>[2x]SDNDPLVVNTDKGRIRGITVDAPSGKKVDVWLGIPYAQPPVGPLRFRHPRPAEKWTGVLNTTTPPNSCVQIVDTVFGDFPGATMWNPNTPLSEDCLYINVVAPRPRPKNAAVMLWIFGGSFYSGTATLDVYDHRALASEENVIVVSLQYRVASLGFLFLGTPEAPGNAGLFDQNLALRWVRDNIHRFGGDPSRVTLFGESAGAVSVSLHLLSALSRDLFQRAILQSGSPTAPWALVSREEATLRALRLAEAVGCPHEPSKLSDAVECLRGKDPHVLVNNEWGTLGICEFPFVPVVDGAFLDETPQRSLASGRFKKTEILTGSNTEEGYYFIIYYLTELLRKEEGVTVTREEFLQAVRELNPYVNGAARQAIVFEYTDWTEPDNPNSNRDALDKMVGDYHFTCNVNEFAQRYAEEGNNVYMYLYTHRSKGNPWPRWTGVMHGDEINYVFGEPLNPTLGYTEDEKDFSRKIMRYWSNFAKTGNPNPNTASSEFPEWPKHTAH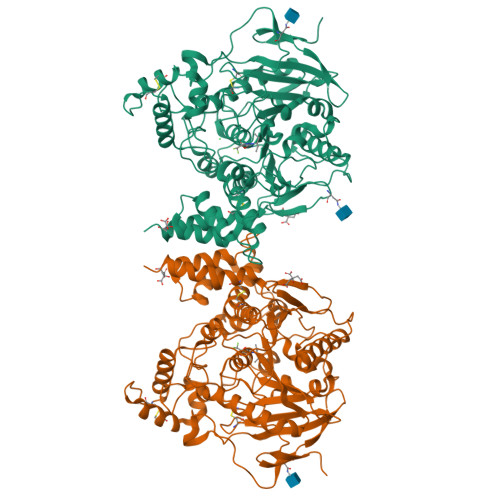GRHYLELGLNTSFVGRGPRLRQCAFWKKYLPQLVAATSNLPG>MKITYIDKPTYLPSWVINKINEYGDFEVFYDFPNEEEAINRLSSTDIAIVEWTSITKEMIEKISRLKYLITITTSYDYIDVNSLKDNEIMVSNCPQYSKQAVAEHVFALLFAVNRKILQADETCRKGLSHIYPPFLCSEIRDKTIGLIGIGQIGQTVAEIANAFQMKVIGLNKSKRNVKGIQQVDITELMKKSDIISLHIPRNADTEIILTEKLLSLMKPDAVLINTCRGNLIDEQALYSVLKQNRIRGAGLDDLTYYKDNPIIGLNNVVLTPGSAWYSYEAREKNMYELIEN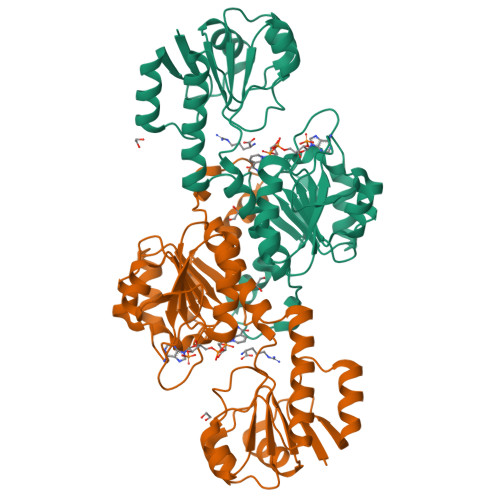IESYLAQKPVNVILEHHHHHH[2x]> MNGTGGAFEGGLFSPYLTTRLPGWAGVRQNVMGSTVD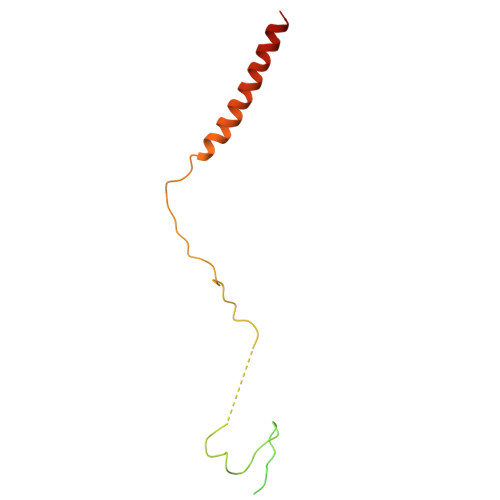GRPVLPANSSTMTYATVGSSSLDSTAAAAAAAAAMTATRLASSYMPSSGSSPSVPSSIIAEEKLLALLAELEALSRQLAALTQQVSELREQQQQQNK>[2x]MENKIEVNSKDEMNKWFEEFKKGNGLVDTYTNSYSFCESVPNLDRFVFQMAGATDDAQKDSIYASALVEATKFCAPIYECAWASSTGIVKKGLEWFEKNTGTIKSWDESYIELKVEVPKIEQLFNYQQAALKWRKDIGFRVNANTAALSNKVLAEYKVPGEIVMSVKEMLSDMIRRRNLILNRGGDENPRGPVSHEHVEWCREFVKGKYIMAFNPPWGDINKSGRSGIALVATGLAKLAETEGKGVFDEAKKTVEALNGYLDKHKDEVDKASADNMVTNLLKHVAKAQELYKNSSALRAQGAQIDTVFSSYYWLYKAGVTPETFPTVSQFLFELGKHPRGTKKMKKALLSTPMKWGKKLYELFADDSFQQNRIYMHPAVLTAGRISEMGVCFGTIPVANPDDAALGSGHTKSILNLRTNTETNNPCARTIVKLFEIQKTGFNIQDMDIVASEHLLHQSLVGKQSPFQNAYNVKGNATSANII;>[2x]ENSLEIEELARFAVDEH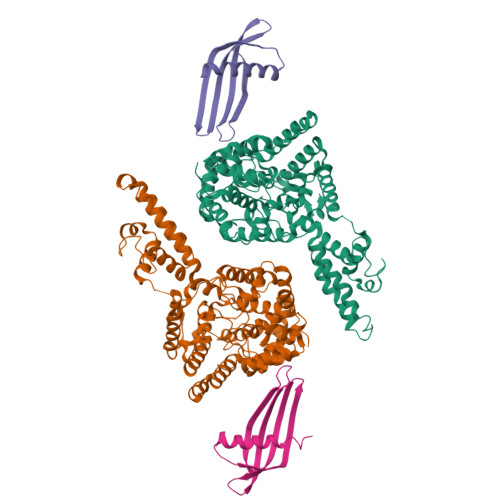NKKENALLEFVRVVKAKEQMHMKERQINTMYYLTLEAKDGGKKKLYEAKVWVKKYLGDFWKDNFKELQEFKPV> MKGTIVGTWIKTLRDLYGNDVVDESLKSVGWEPDRVITPLEDIDDDEVRRIFAKVSEKTGKNVNEIWREVGRQNIKTFSEWFPSYFAGRRLVNFLMMMDEVHLQLTKMIKGATPPRLIAKPVAKDAIEMEYVSKRKMYDYFLGLIEGSSKFFKEEISVEEVERGEKDGFSRLKVRIKFK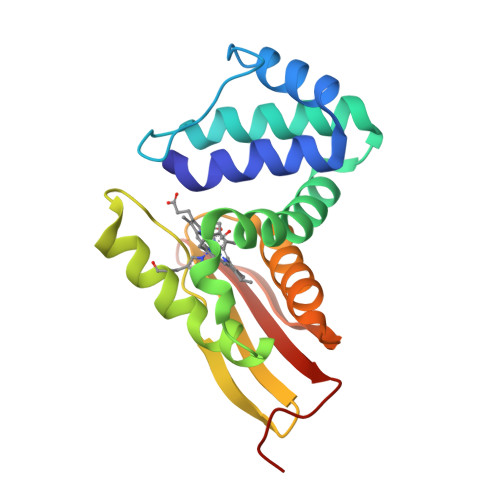NPVFEYKKN>MTQVAEIKSPHEQRLEDNIAGKEDIYRESHKRVFKLLERFDGQKPAIDVERALYFTQSMAETVGQPLVLRWAKALMNVAKNITVMVQDDQLLLGRCGGHDGRYGILYPELDGDFLDIAVRDLPTRPQSPASISPEDAKIVVEQIAPFWKGRTYHEALNKALPAEVHKLTYDDPDGLISRFIVNETSSFRSSIQWVHDYEVVLKRGFNGLKQEMEEKLAALDPASPVDQVDKRPFIEATILVCDAIVLWAKRHADAARKAAEACADPVRKAELIRMAENAEHVPANPARDFYEAVQSQYFTQMFSRLEQKTGTTISNGRMDQYFYPFYKKDMEAGILTDEKTLEYLECMWVGMAEFIDMYISPAGGAFNEGYAHWEAVTIGGQTPDGRDATNDLTYLFLKSKREFPLHYPDLAARIHSRAPERYLWDVAETIKFGSGFPKLCNDEECIPLYVSKGATFEEALDYAVSGCIEIRMPNRDTYTSGGAYTNFASAVEMALYDGKMKKYGDVQLGIQTGDARKFKSWDEFWNAYVQQHMLLLRTTFIQQYIVIQTRAKHFAQPMGSVLHALCRKHCIDL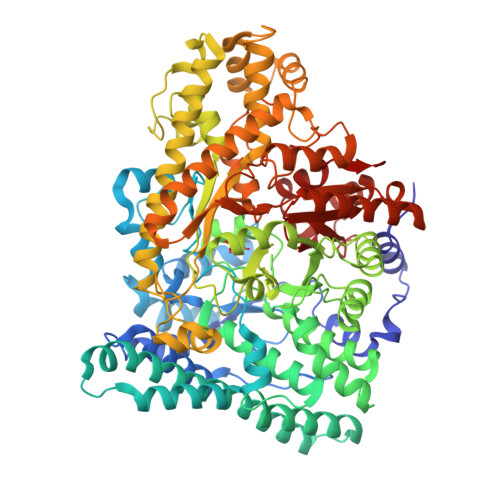HQPQIPEGLNFGYFEFMGLGTVIDSLAAIKKLVFEDKKLTMDQLIDALEANFEGYEDIQQLLRTAPCYGNDDEYADEIGRELDRMAVSFAAKYGKEMGINNDARYVPFTSHVPFGKVVSATPNGRVAWFPLADGSSPSHGADHNGPTAILLSNHNTKNYGMRARAARLINVKFTPKCVEGDAGTEKLVQFIRTWCDLKLWHIQFNVINADTLKKAQKDPQKYRNLIVRIAGYSAYFVDLTPDLQNDLIARTGHDQM[4x]> GGGG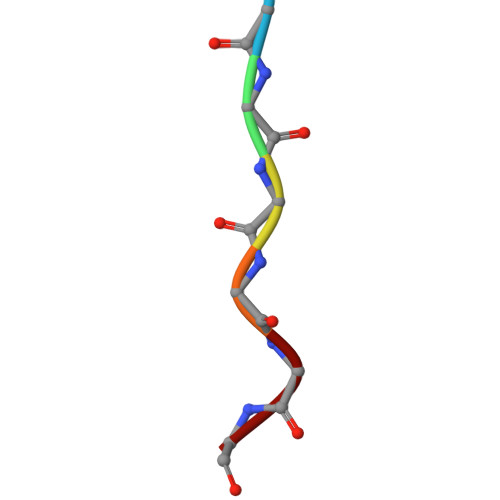GG> TIQNDIPDLYSVFKDYFPIGVAVDPSRLNDADPHAQLTAKHFNMLVAENAMKPESLQPTEGNFTFDNADKIVDYAIAHNMKMRGHTLLWHNQVPDWFFQDPSDPSKPASRDLLLQRLRTHITTVLDHFKTKYGSQNPIIGWDVVNEVLDDNGNLRNSKWLQIIGPDYIEKAFEYAHEADPSMKLFINDYNIENNGVKTQAMYDLVKKLKNEGVPINGIGMQMHISINSNIDNIKASIEKLASLGVEIQVTELDMNMNGDVSNDALLKQARLYKQLFDLFKAEKQYITAVVF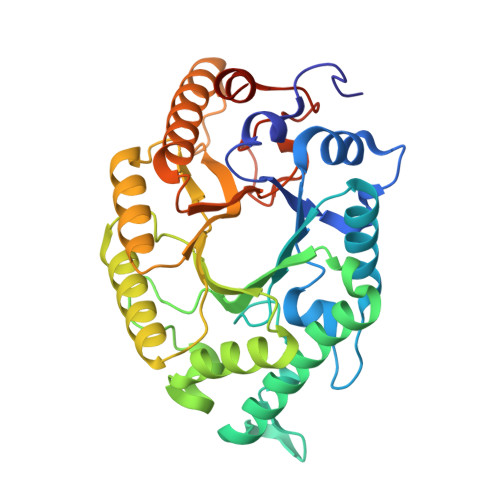WGVSDDVSWLSKPNAPLLFDSKLQAKPAYWAIVDLGKAIPDIQSA> GSHMNAPENYIR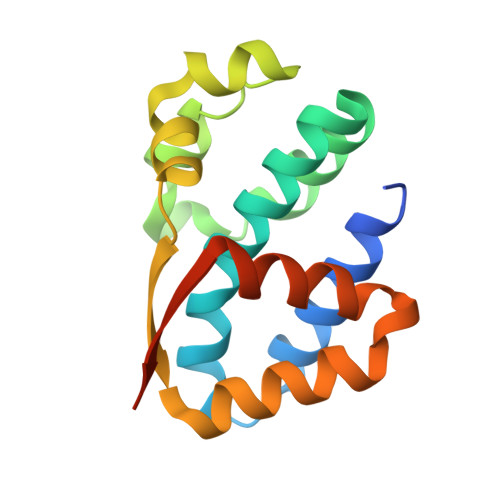AYSMLKNWVDSSLEIYKPELSYIMYPIFIYLFLNLVAKNPVYARRFFDRFSPDFKDFHGSEINRLFSVNSIDHIKENEVASAFQSHKYRITMSKTTLNLLLYFLNENESIGGSLIISVINQHLDPNIVESVTAREK We identified two virulence pili independently critical to A. baumannii catheter-associated urinary tract infections, the chaperone-usher pathway pili Abp1 and Abp2. Further, their respective tip-adhesive proteins, the adhesins Abp1D and Abp2D, make use of large, distally oriented binding pockets to adhere to glycoproteins like fibrinogen, a wound-healing protein important in CAUTI pathogenesis. We demonstrate that Abp1D and Abp2D RBDs are structurally similar, and each binds fibrinogen and other relevant host glycoproteins important in CAUTI and other infections. These proteins share a common binding mechanism, using a large, distally oriented, and flexible pocket that recognizes a complex glycan receptor.

When determining the Abp1DRBD structure, we solved two molecules of this protein in the crystal (asymmetric) unit. The structures of the two molecules of Abp1DRBD had a backbone rmsd value of 0.176 Å, demonstrating that they are highly similar. However, while most of the binding pocket was structurally conserved, one region of substantial variation was a 10 amino acid stretch (R86-S95) encompassing the anterior binding pocket loop. Compared to molecule A Abp1DRBD, molecule B’s anterior binding pocket loop was displaced up and into the pocket, moving the α-carbon of S91 by 7.9 Å in the >50 Å long structure. The rmsd value of the backbone of this region was 2.275 Å, indicating that it was substantially distorted from one Abp1DRBD molecule to another. The anterior loop’s flexibility is significant because this loop can change the shape of the binding pocket, which likely affects protein function. While these two residues are conserved in the Abp1DRBD, they are too far away from each other (>4 Å) (in the crystal structures) to form a salt bridge in both Abp1DRBD molecule A or Abp1DRBD molecule B and the loops are more closed than in the Abp2DRBD structure (especially in molecule B of the Abp1DRBD structure). An R86E variant of Abp1DRBD similarly abolished binding to BSM as measured by enzyme-linked immunosorbent assay (ELISA). Though Abp1D and Abp2DACICU share residues critical for adherence (R86, R102, and Y141), Abp2DRBD has a higher affinity for fibrinogen than Abp1DRBD.

>[2x]NCTLSKGFTTVDIPMTIGTIVVRPTDPIGTVLQKNTFTISPNNSTATCNRASDQITAALPLNYPVSSIGNNVYATNIPGIGIRLYREAFDSTDFSGYYPYKRSLTPNTTYTLSPGYFVMEVIKTAATTGSGALVAGRYSTYYVTGQQNRPFLTTTVLSSSPILIASSSHHHHHH4-[2-(3-BENZYLOXYCARBONYLAMINO-4-CYCLOHEXYL-1-HYDROXY-2-OXO-BUTYLAMINO)-5-GUANIDINO-PENTANOYLAMINO]-4-(1-CARBOXY-2-CYCLOHEXYL-ETHYLCARBAMOYL)-BUTYRIC 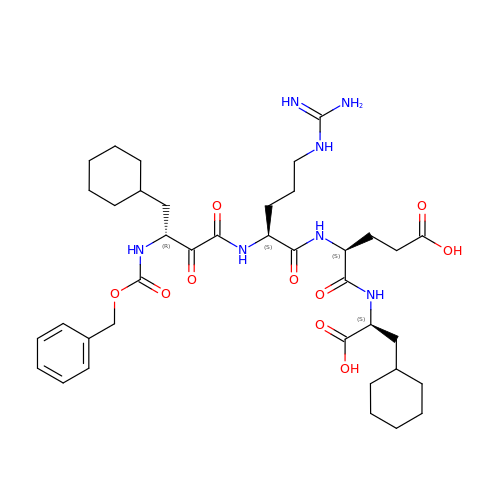ACID | C38 H57 N7 O10 | LKCWMWZIRUHWBW-ZXYZSCNASA-N> GPAFEFAVAMMKRNSSTVKTEYGEFTMLGIYDRWAVLPRHAKPGPTILMNDQEVGVLDAKELVDKDGTNLELTLLKLNRNEKFRDIRGFLAKEEVEVNEAVLAINTSKFPNMYIPVGQVTEYGFLNLGGTPTKRMLMYNFPTRAGQCGGVLMSTGKVLGIHVGGN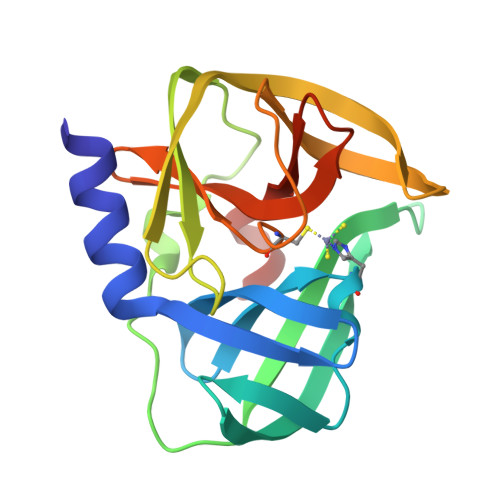GHQGFSAALLKHYFNDEQ> MGYTRERTNRHFFVARANAFFSRLPIARVQRSLAMEAVREGRMRPWKYTKEQILGAPVTCNFEYNPRPVRLIG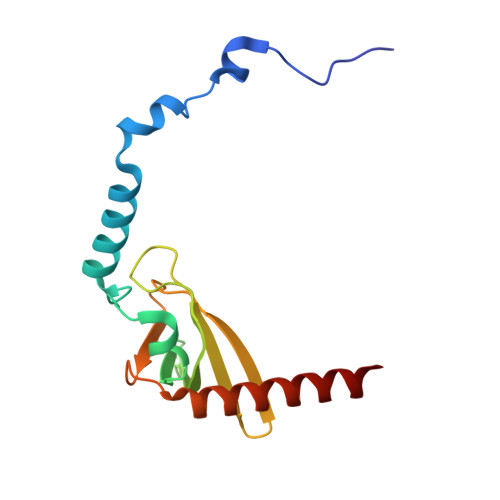TVMDAHTEETSIKGGLKVYARNEETNMMLWIPPGNPKLRHEVTSTKGSFQHYLDERDKWDEAWITGRARMK> MRPSAIVLAGGKEAWAERFGVGSKALVPYRGRPMVEWVLEALYAAGLSPVYVGENPGLVPAPALTLPDRGGLLENLEQALEHVEGRVLVATGDIPHLTEEAVRFVLDKAPEAALVYPIVPKEAVEARFPRTKRTYARLREGTFTGGNLLLLDKSLFRKALPLARRVVALRKRPLALARLVGWDVLLKLLLGR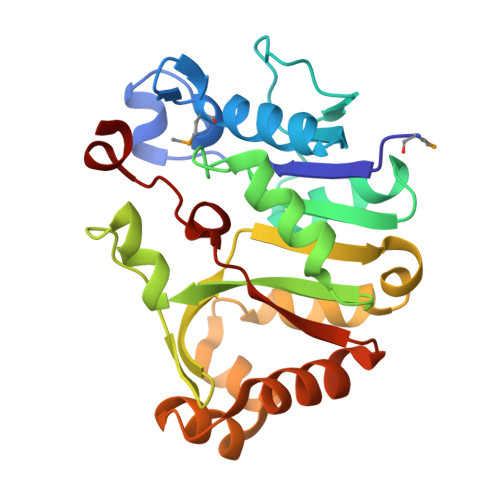LSLAEVEARAQRILGVEARALVTPYPEVGVDVDREEDLVS2-chloro-5-{[(2E)-2-(nitromethylidene)imidazolidin-1-yl]methyl}pyridine 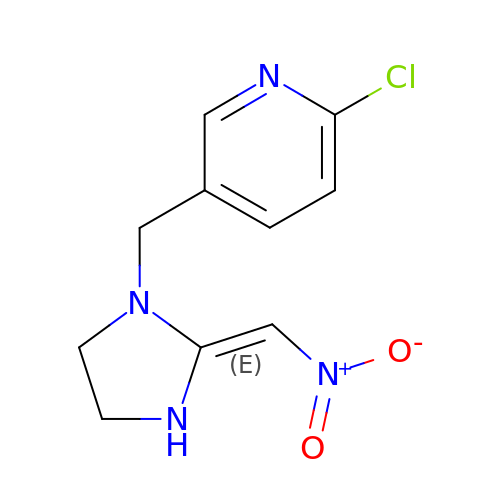| C10 H11 Cl N4 O2 | ALNDHUQPXHHNON-JXMROGBWSA-N>[4x]SNAMNKTELIKNVAQNAEISQKEATVVVQTVVESITNTLAAGEKVQLIGFGTFE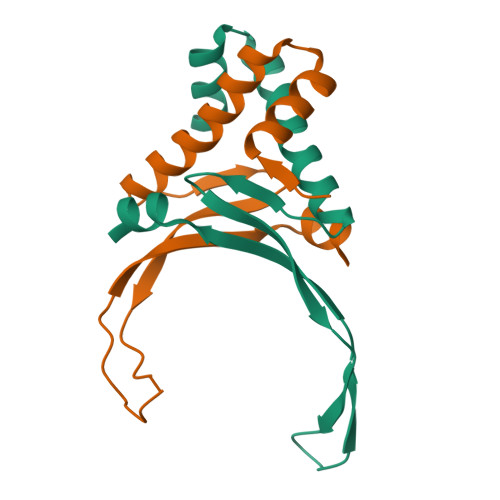VRERAARTGRNPQTGEEMQIAASKVPAFKAGKELKEAVK> MLRRTIVPLAKVYGAAPPNGTGQMQPARHRLLHGKRERQGSLFAIANDVKYDEKRLRQQLNAMLEEERLPPRTRLERNKANGGEALPQRRLVDLPGVERRRDLPADPITRLFFQHKGDHALYYGTYDNPSLQDEDRIQIEKREPRYWTYNVFTPVYDFCHRIREATEQRKRFVIVPSTVETRGCARVMLGHGLVAGFRDFHNDRAFAVELKYFQGDSTINVIEPCAYDGKTEFEWSPKMMRRLMNTHGIHNRLVVY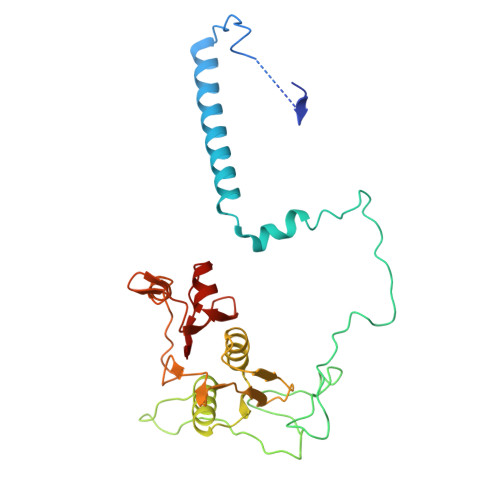ICRTADNRVIDHIQAVKENVGGRGLIMVH> 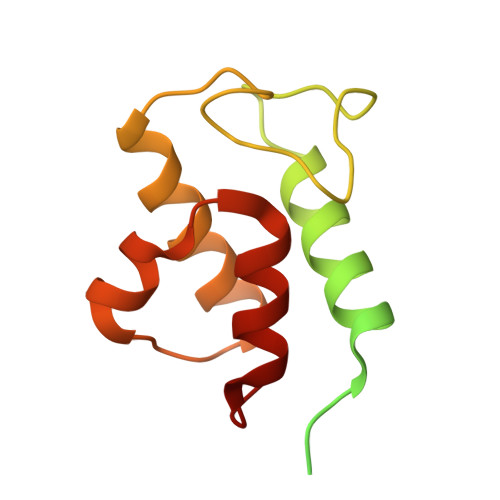MQRSQLARKFATQVGAYSLLRGRCHAVSTWKVMATQAVTIPMYLPVRFHSEGHAAGEEAGRTGQYLLNKDDVLTRVLEVVKNFEKVDASKVTPQSHFVNDLGLNSLDVVEVVFAIEQEFILDIPDHDAEKIQSITDAVEYISQNPMAK>RAPDSVDYRKKGYVTPVKNQGQCGSCWAFSSVGALEGQLKKKTGKLLNLSPQNLVDCVSENDGCGGGYMTNAFQYVQKNRGIDSEDAYPYVGQEESCMYNPTGKAAKCRGYREIPEGNEKALKRAVARVGPVSVAIDASLTSFQFYSKGVY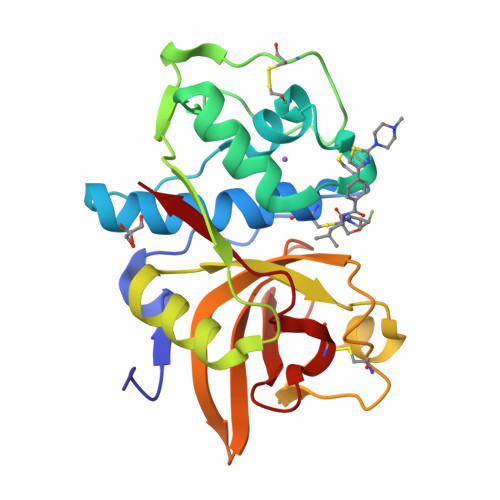YDESCNSDNLNHAVLAVGYGIQKGNKHWIIKNSWGENWGNKGYILMARNKNNACGIANLASFPKM[2x]> HPETLVKVKDAEDQLGARVGYIELDLNSGKILESFRPEERFPMMSTFKVLLCGAVLSRVDAGQEQLGRRIHYSQRDLVEYSPVTEKHLTDGMTVRELCSAAITMSDNTAANLLLTTIGGPKELTAFLHNMGDHVTRLDRWEPELNEAIPNDERDTTMPAAMATTLRKLLTGELLTLASRQQLIDWMEADKVAGPLL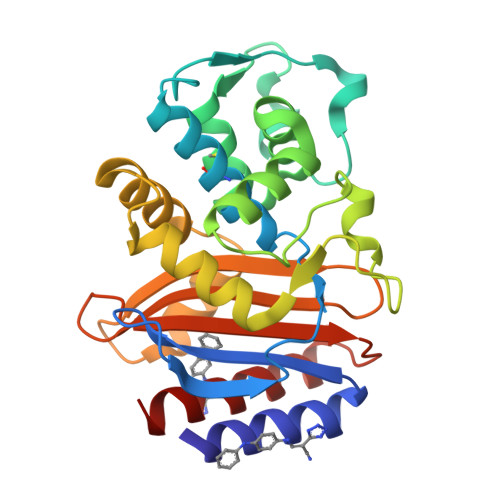RSALPAGWFIADKSGAGERGSRGIIAALGPDGKPSRIVVIYTTGSQATMDERNRQIAEIGASLIKHW> MELHQIRGCHKNDIELKKYNIGVAISLGNKWFSIDNIEKLVKWSLLHTKEYVIIYIADSIHGINLSVRNKLSDSHAEEVAIRYGRNLFIKIKERVSLSFSQDEQAKIIYATWSDIADSKYKEKVKYLYNLYDKNINFKNYIENFVKEWVSKEKRTFNNNE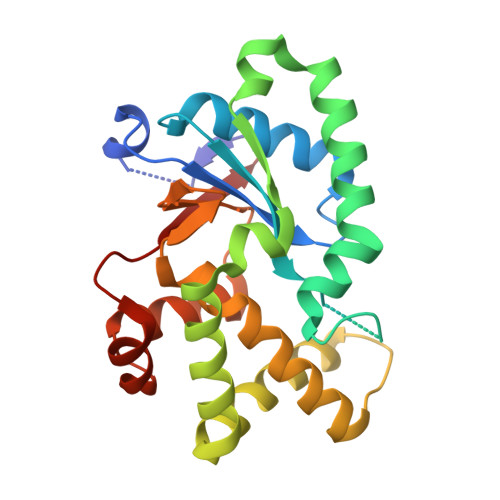INKFGRYILEELPALMVQVKARGVLFEAYVYPYKTRITEFVGLLQKGEIFPEIKTNILDNHPKIFLEVRE>[4x]SATLFNNIELLPPDALFGIKQRYGQDQRATKVDLGIGAYRDDNGKPWVLPSVKAAEKLIHNDSSYNHEYLGITGLPSLTSNAAKIIFGTQSDALQEDRVISVQSLSGTGALHISAKFFSKFFPDKLVYLSKPTWANHMAIFENQGLKTAT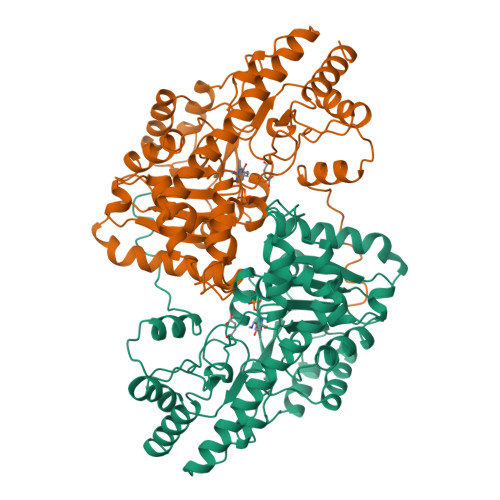YPYWANETKSLDLNGFLNAIQKAPEGSIFVLHSCAHNPTGLDPTSEQWVQIVDAIASKNHIALFDTAYQGFATGDLDKDAYAVRLGVEKLSTVSPVFVCQSFAKNAGMYGERVGCFHLALTKQAQNKTIKPAVTSQLAKIIRSEVSNPPAYGAKIVAKLLETPELTEQWHKDMVTMSSRITKMRHALRDHLVKLGTPGNWDHIVNQCGMFSFTGLTPQMVKRLEETHAVYLVASGRASIAGLNQGNVEYVAKAIDEVVRFYA>QPVRYSIPEELDRGSVVGKLAKDLGLSVLEVSARKLRVSAEKLHFSVDSESGDLLVKDRIDREQICKGRRKCELQLEAVLENPLNIFHVVVEIEDVNDHAPQFPKDEINLEISESDSPGARTILESAKDLDIGMNSLSKYQLSPNDYFLLLVKDNPDGSKYPELELQKMLDREAESTHHLMLTAVDGGDPPRTGTTQLRIRVVDANDNRPVFSQDVYRVRLPEDLPPGTTVLRLKAMDQDEGINAEFTYSFLGVANKAQFSLDPITGDIVTRQSLDFEEVEQYTIDVEAKDRGSLSSQCKVIIEVLDENDNRPEIIITSLSDQISEDSPSGTVVALFKVRDRDSGENAEVMCSLSGNNPFKIHSSSNNYYKLVTDSILDREQTPGYNVTITATDRGKPPLSSSTTITLNVADVNDHHHHH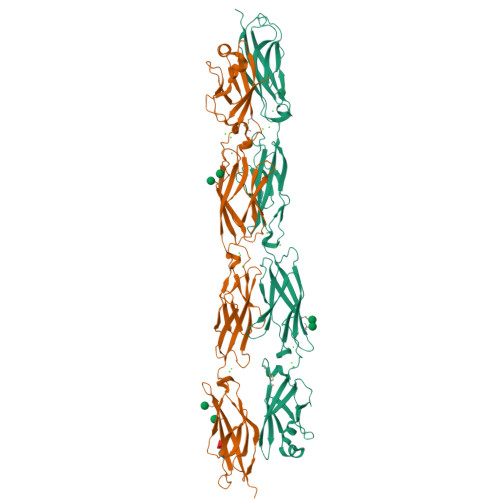HHH[2x]> QPESLRPVNLTQERNILPMTPVWAPVPNLNADLKKLNCSPDSFRCTLTNIPQTQALLNKAKLPLGLLLHPFRDLTQLPVITSNTIVRCRSCRTYINPFVSFIDQRRWKCNLCYRVNDVPEEFMYNPLTRSYGEPHKRPEVQNSTVEFIASSDYMLRPPQPAVYLFVLDVSHNAVEAGYLTILCQSLLENLDKLPGDSRTRIGFMTFDSTIHFYNLQEGLSQPQMLIVSDIDDVFLPTPDSLLVNLYESKELIKDLLNALPNMFTNTRETHSALGPALQAAFKLMSPTGGRVSVFQTQLPSLGAGLLQSREDPNQRSSTKVVQHLGPATDFYKKLALDCSGQQTAVDLFLLSSQYSDLASLACMSKYSAGCIYYYPSFHYTHNPSQAEKLQKDLKRYLTRKIGFEAVMRIRCTKGLSMHTFHGNFFVRSTDLLSLANINPDAGFAVQLSIEESLTDTSLVCFQTALLYTSSKGERRIRVHTLCLPVVSSLADVYAGVDVQAAICLLANMAVDRSVSSSLSDARDALVNAVVDSLSAYGSTVSNLQHSALMAPSSLKLFPLYVLALLKQKAFRTGTSTRLDDRVYAMCQIKSQPLVHLMKMIHPNLYRIDRLTDEGAVHVNDRIVPQPPLQKLSAEKLTREGAFLMDCGSVFYIWVGKGCDNNF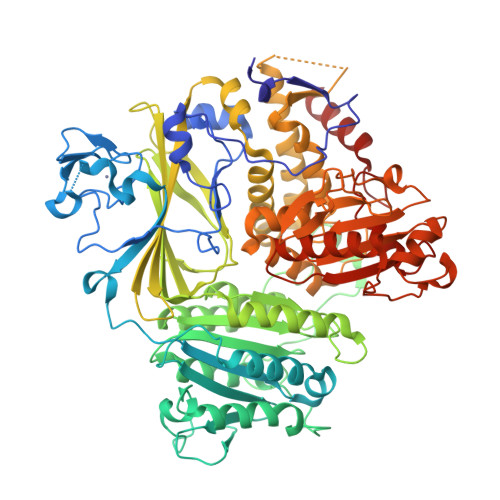IEDVLGYTNFASIPQKMTHLPELDTLSSERARSFITWLRDSRPLSPILHIVKDESPAKAEFFQHLIEDRTEAAFSYYEFLLHVQQQICK> MKTITTFENKKVLVLGLARSGEAAARLLAKLGAIVTVNDGKPFDENPTAQSLLEEGIKVVCGSHPLELLDEDFCYMIKNPGIPYNNPMVKKALEKQIPVLTEVELAYLVSESQLIGITGSNGKTTTTTMIAEVLNAGGQRGLLAGNIGFPASEVVQAANDKDTLVMELSSFQLMGVKEFRPHIAVITNLMPTHLDYHGSFEDYVAAKWNIQNQMSSSDFLVLNFNQGISKELAKTTKATIVPFSTTEKVDGAYVQDKQLFYKGENIMSVDDIGVPGSHNVENALATIAVAKLAGISNQVIRETLSNFGGVKHRLQSLGKVHGISFYNDSKSTNILATQKALSGFDNTKVILIAGGLDRGNEFDELIPDITGLKHMVVLGESASRVKRAAQKAGVTYSDA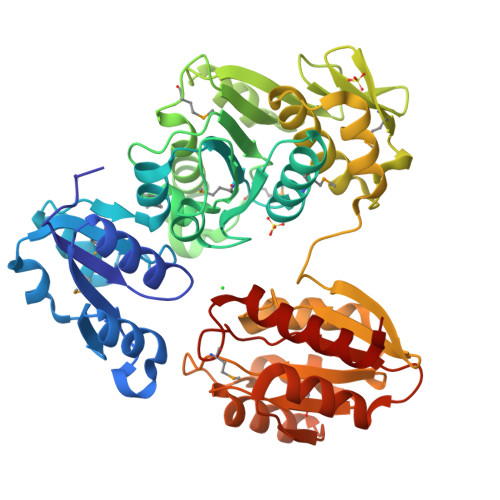LDVRDAVHKAYEVAQQGDVILLSPANASWDMYKNFEVRGDEFIDTFESLRGE(2E)-3-{5-[(2,4-diaminopyrimidin-5-yl)methyl]-2,3-dimethoxyphenyl}-1-[(1S)-1-(2-methylpropyl)phthalazin-2(1H)-yl]prop-2-en-1-one 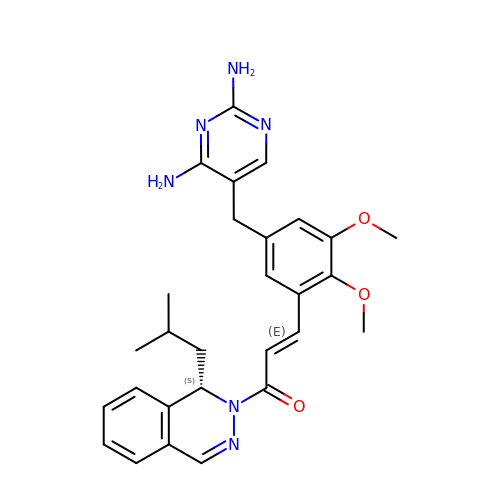| C28 H32 N6 O3 | ZISYTWICFLBNJQ-ZUTVHTERSA-N> SMENKNLNYILGLDLGIASVGWAVVEIDEKENPLRLIDVGVRTFERAEVPKTGESLALSRRLARSARRLTQRRVARLKKAKRLLKSENILLSTDERLPHQVWQLRVEGLDHKLERQEWAAVLLHLIKHRGYLSQRKNESKSENKELGALLSGVDNNHKLLQQATYRSPAELAVKKFEVEEGHIRNQQGAYTHTFSRLDLLAEMELLFSRQQHFGNPFASEKLLENLTALLMWQKPALSGEAILKMLGKCTFEDEYKAAKNTYSAERFVWITKLNNLRIQENGLERALNDNERLALMEQPYDKNRLFYSQVRSILKLSDEAIFKGLRYSGEDKKAIETKAVLMEMKAYHQIRKVLEGNNLKAEWAELKANPTLLDEIGTAFSLYKTDEDISAYLAGKLSQPVLNALLENLSFDKFIQLSLKALYKLLPLMQQGLRYDEACREIYGDHYGKKTEENHHFLPQIPADEIRNPVVLRTLTQARKVINGVVRLYGSPARIHIETGREVGKSYKDRRELEKRQEENRKQRENAIKEFKEYFPHFAGEPKAKDILKMRLYKQQNAKCLYSGKPIELHRLLEKGYVEVDHALPFSRTWDDSFNNKVLVLANENQNKGNLTPFEWLDGKHNSERWRAFKALVETSAFPYAKKQRILSQKLDEKGFIERNLNDTRYVARFLCNFIADNMHLTGEGKRKVFASNGQITALLRSRWGLAKSREDNDRHHALDAVVVACSTVAMQQKITRFVRFEAGDVFTGERIDRETGEIIPLHFPTPWQFFKQEVEIRIFSDNPKLELENRLPDRPQANHEFVQPLFVSRMPTRKMTGQGHMETVKSAKRLNEGISVIKMPLTKLKLKDLELMVNREREKDLYDTLKARLEAFNDDPAKAFAEPFIKKGGA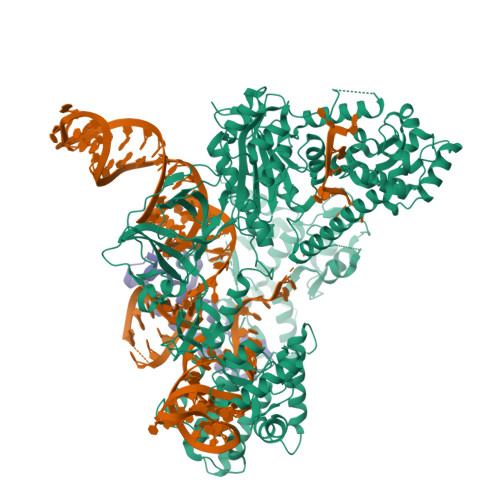IVKSVRVEQIQKSGVLVREGNGVADNASMVRVDVFTKGGKYFLVPIYTWQVAKGILPNKAATQYKDEEDWEVMDNSATFKFSLHPNDLVKLVTKKKTILGYFNGLNRATGNIDIKEHDLDKSKGKQGIFEGVGIKLALSFEKYQVDELGKNIRLCKPSKRQPVR;> SMKITSSNFATIATSENFAKLSVLPKNHREPIKGLFKSAVEQFSSARDFFKNENYSKELAEKFNKEAVNEAVEKLQKAIDLAEKQGIQF> KSCCRSTLGRNCYNLCRARGAQKLC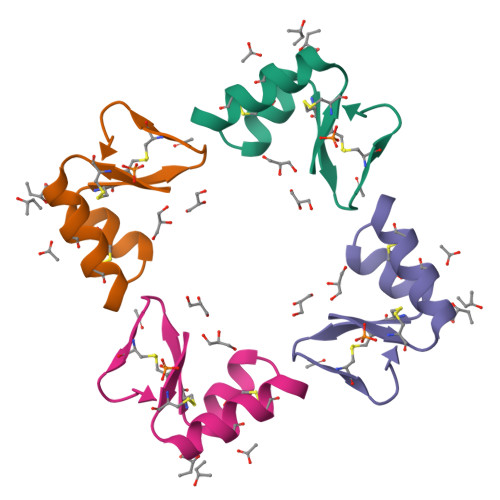AGVCRCKISSGLSCPKGFPK> MKKTQRKEIENVTNITGVRQIELWRRDDLQHPRLDEVAEEVPVALVYNGISHVVMMASPKDLEYFALGFSLSEGIIESPRDIFGMDVVPSCNGLEVQIELSSRRFMGLKERRRALAGRTGCGVCGVEQLNDIGKPVQPLPFTQTFDLNKLDDALRHLNDFQPVGQLTGCTHAAAWMLPSGELVGGHEDVGRHVALDKLLGRRSQEGESWQQGAVLVSSRASYEMVQKSAMCGVEILFAVSAATTLAVEVAERCNLTLVGFCKPGRATVYTHPQRLS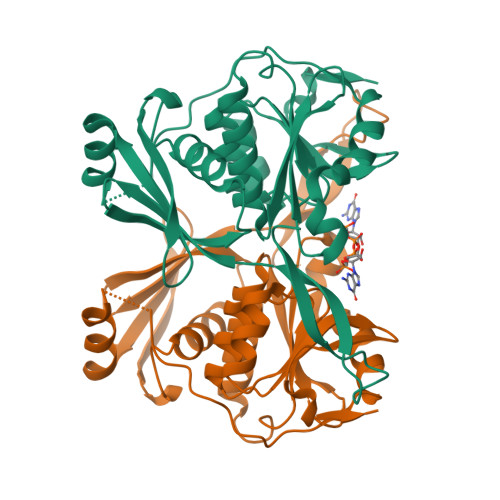NLEHHHHHH> TTHFSIVDKDGNAVSNTYTLNWDFGSGVVVKGAGFLLNDEMDDFSSKPG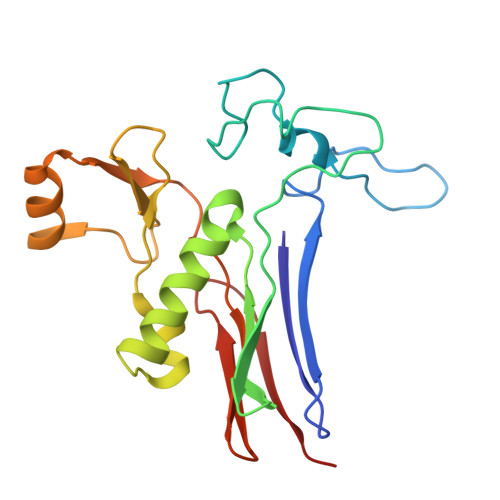VANAFGVVGSDANAIEPGKRMLSSMSPSIVTRDGHVSLVLGTPGGSRIFTSIFQVLNNVYDFHLPLEKAVAAQRVHHQLLPKDTIYYDAYAPLTGKVADELKAMGYTLEDQGWNMGDIQAIRVNGKALETASDPRGRGVGMVVKP>[2x]GPLGSMLNPQLVQPAKKPYNKIVSHLLVAEPEKIYAMPDPTVPDSDIKALTTLCDLADRELVVIIGWAKHIPGFSTLSLADQMSLLQSAWMEIL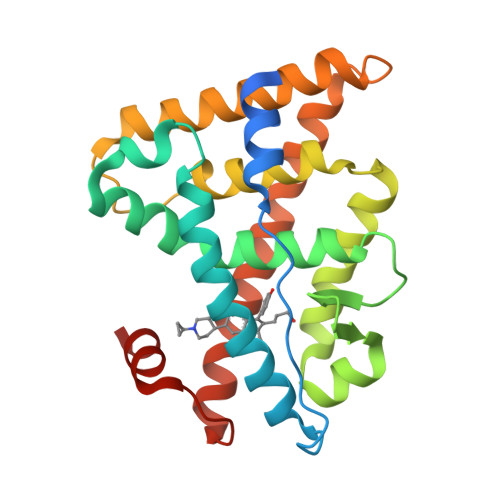ILGVVYRSLSFEDELVYADDYIMDEDQSKLAGLLDLNNAILQLVKKYKSMKLEKEEFVTLKAIALANSDSMHIEDVEAVQKLQDVLHEALQDYEAGQHMEDPRRAGKMLMTLPLLRQTSTKAVQHFYNIKLEGKVPMHKLFLEMLEAKV> MGVVEEAHNVKVIGSGEATIVLGHGFGTDQSVWKHLVPHLVDDYRVVLYDNMGAGTTNPDYFDFDRYSNLEGYSFDLIAILEDLKIESCIFVGHSVSAMIGVLASLNRPDLFSKIVMISASPRYVNDVDYQGGFEQEDLNQLFEAIRSNYKAWCLGFAPLAVGGDMDSIAVQEFSRTLFNMRPDIALSVGQTIFQSDMRQILPFVTVPCHILQSVKDLAVPVVVSEYLHANLGCESVVEVIPSDGHLPQLSSPDSVIPVILRHIRNDIAM

A few components involved in KAR-signaling have been identified in Arabidopsis thaliana, including an α/β hydrolase fold protein, KARRIKIN INSENSITIVE2/HYPOSENSITIVE TO LIGHT (hereafter referred to as KAI2), an F-box protein, MORE AXILLARY GROWTH2 (MAX2, also referred to as ORESARA9/PLEIOTROPIC PHOTO SIGNALING/KARRIKIN INSENSITIVE1), and SUPPRESSOR OF MAX2 1 (SMAX1)/SMAX1-LIKE2 (SMXL2). Crystallographic studies and biochemical analyses have demonstrated the role of KAI2 as a KAR receptor. The structure of KAI2 displayed a canonical compact α/β-hydrolase domain that contained an α/β ‘core’ domain and a ‘lid’ domain. A smoke-derived compound, karrikin (KAR), and an endogenous but as yet unidentified KARRIKIN INSENSITIVE2 (KAI2) ligand (KL) have been identified as chemical cues in higher plants that impact on multiple aspects of growth and development.

Recombinant proteins of KAI2 and KAI2ply2, purified from E. coli, were crystallized. Comparison of KAI2 and KAI2ply2 showed that there was little structural difference (r.m.s.d., 0.2 Å) in overall structure. However, in detail, we found that the residue A219 of KAI2 was bound to aromatic residues as Y124 and F134 of the lid domain by hydrophobic interactions, while the residue V219 of KAI2ply2 was bound to extended aromatic residues as Y124, F134, F157, F194, and H246 of the lid domain. The entrance of KAI2 presents an opened pocket and hydrophobic charge for the ligand, whereas the entrance of KAI2ply2 forms a closed pocket due to C-gamma 1 and C-gamma 2 of V219, which is a bulkier residue than alanine. The results showed that the amino acid residues of KAI2 ranging from 125–150 exhibited a higher B-factor than those of KAI2ply2, implying that this region, corresponding to the helical ‘lid’ domain, might be more rigid with lower motional amplitude in the KAI2ply2 protein. We found that the Tm of the KAI2ply2 protein was increased compared to that of the wild-type KAI2 under CD assay conditions; the Tm values of KAI2 and KAI2ply2 were calculated to be 45.23 °C and 49.36 °C, respectively. Thus, the Ala219 of KAI2 appears to be important in forming space for entry of the ligand as well as maintaining flexibility of the lid domain.> GAMAKVQVNNVVVLDNPSPFYNPFQFEITFECIEDLSEDLEWKIIYVGSAESE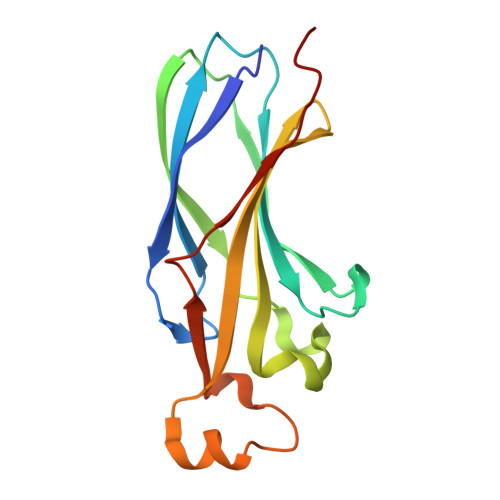EYDQVLDSVLVGPVPAGRHMFVFQADAPNPGLIPDADAVGVTVVLITCTYRGQEFIRVGYYVNNEYTETELRENPPVKPDFSKLQRNILASNPRVTRFHINWEDN> STGSATTTPIDSLDDAYITPVQIGTPAQTLNLDFDTGSSDLWVFSSETTASEVDGQ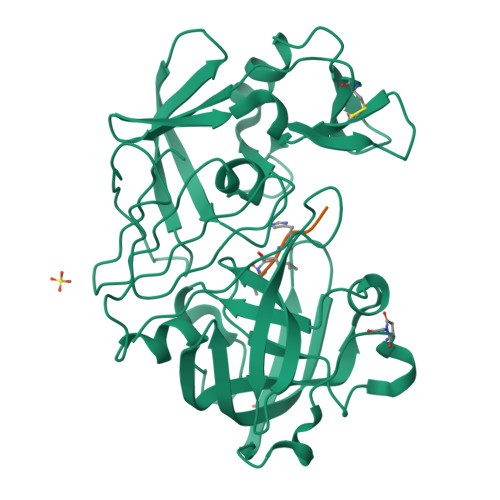TIYTPSKSTTAKLLSGATWSISYGDGSSSSGDVYTDTVSVGGLTVTGQAVESAKKVSSSFTEDSTIDGLLGLAFSTLNTVSPTQQKTFFDNAKASLDSPVFTADLGYHAPGTYNFGFIDTTAYTGSITYTAVSTKQGFWEWTSTGYAVGSGTFKSTSIDGIADTGTTLLYLPATVVSAYWAQVSGAKSSSSVGGYVFPCSATLPSFTFGVGSARIVIPGDYIDFGPISTGSSSCFGGIQSSAGIGINIFGDVALKAAFVVFNGATTPTLGFASK;> PHPFHXVIHK>[3x]MISNNAPAKMVLNSVLTGYTLAYIQH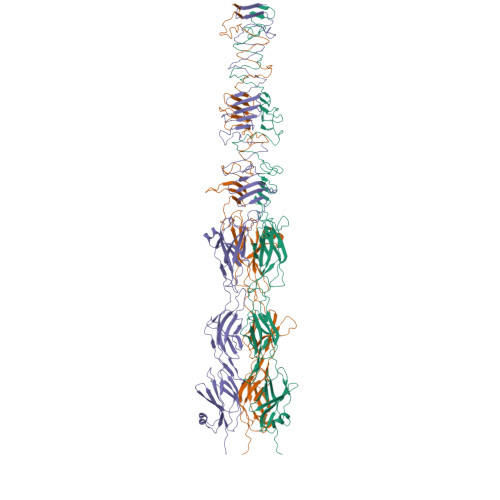SIYSDYDVIGRSFWLKEGSNVTRRDFTGIDTFSVTINNLKPTTTYEVQGAFYDSIIDSELLNAQIGINLSDKQTFKMKSAPRITGARCESEPVDVGVGAPIVYIDTTGEADYCTIELKDNSNANNPWVKYYVGALMPTIMFGGVPIGSYKVRISGQISLPDGVTIDSSGYYEYPNVFEVRYNFVPPAAPINIVFKAARIADGKERYDLRVQWDWNRGAGANVREFVLSYIDSAEFVRTGWTKAQKINVGAAQSATIISFPWKVEHKFKVSSIAWGPDAQDVTDSAVQTFILNESTPLDNSFVNETGIEVNYAYIKGKIKDGSTWKQTFLIDAATGAINIGLLDAEGKAPISFDPVKKIVNVDGSVITKTINAANFVMTNLTGQDNPAIYTQGKTWGDTKSGIWMGMDNVTAKPKLDIGNATQYIRYDGNILRISSEVVIGTPNGDIDIQTGIQGKQTVFIYIIGTSLPAKPTSPAYPPSGWSKTPPNRTSNTQNIYCSTGTLDPVTNQLVSGTSWSDVVQWSGTEGVDGRPGATGQRGPGMYSLAIANLTAWNDSQANSFFTSNFGSGPVKYDVLTEYKSGAPGTAFTRQWNGSAWTSPAMVLHGDMIVNGTVTASKIVANNAFLSQIGVNIIYDRAAALSSNPEGSYKMKIDLQNGYIHIR> X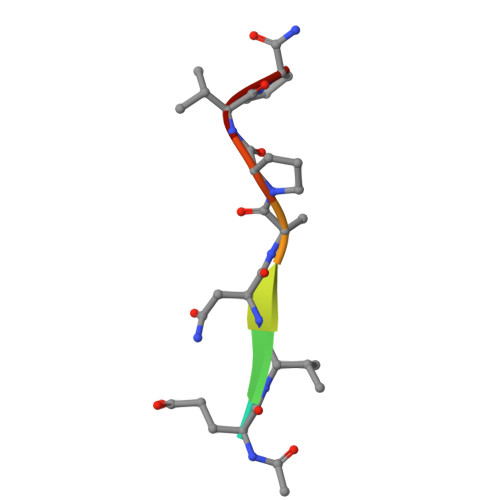EVNAPVP>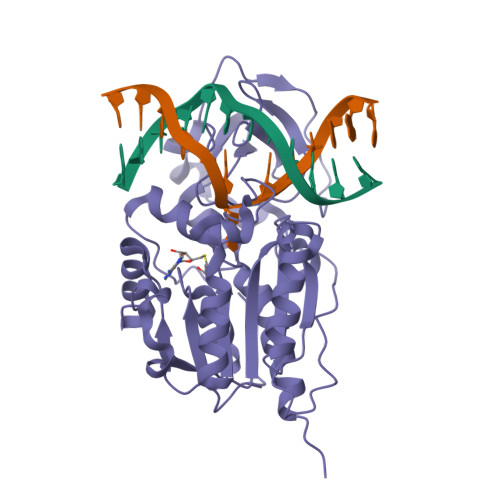 MIEIKDKQLTGLRFIDLFAGLGGFRLALESCGAECVYSNEWDKYAQEVYEMNFGEKPEGDITQVNEKTIPDHDILCAGFPAQAFSISGKQKGFEDSRGTLFFDIARIVREKKPKVVFMENVKNFASHDNGNTLEVVKNTMNELDYSFHAKVLNALDYGIPQKRERIYMICFRNDLNIQNFQFPKPFELNTFVKDLLLPDSEVEHLVIDRKDLVMTNQEIEQTTPKTVRLGIVGKGGQGERIYSTRGIAITLSAYGGGIFAKTGGYLVNGKTRKLHPRECARVMGYPDSYKVHPSTSQAYKQFGNSVVINVLQYIAYNIGSSLNFKPY> MVAESNSAVAPTANVATSPAHEHFVRVNGGHFELQGKPYVITGVNMWYAAYLGAPNEVGDRDRLAKELDNLKAIGVNNLRVLAVSEKSEINSAVKPAVTNGFGNYDETLLQGLDYLLVELAKRDMTVVLYFNNFWQWSGGMTQYMAWIEGEPVQDPNVTNEWEAFMAKSASFYRSEKAQQEYRKTLEKIITRVNSINGKAYVDDATIMSWQLANEPRPGNSQTTAEEKQIYIDWVHAAAAYIKTLDAHHLVSSGS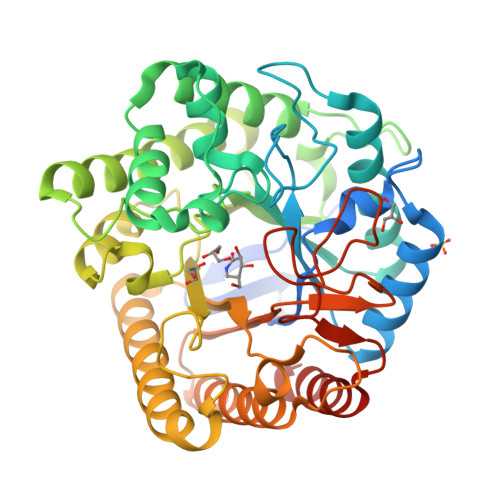EGEMGSVNDMQVFIDAHATPDIDYLTYHMWIRNWSWFDKTKPAETWPSAWEKAQNYMRAHIDVAKQLNKPLVLEEFGLDRDMGSYAMDSTTEYRDNYFRGVFELMLASLEQGEPSAGYNIWAWNGYGRTTRANYWWQEGDDFMGDPPQEEQGMYGVFDTDTSTIAIMKEFNARFQPKLEHHHHHH> MIRIKDFNHVITGREQPLDINEAIASYITSRYVYFKDARRVAEETWLEAWSLYSGTPEAVDHQRTQTINTVGEVNNDWRHRLNTGKAYECIETVHGYLMGALFPNREWFDLTPNNPGYANEARIIRKYLTKKFNEGKFRVSFEKYLRQLLVCGYSVMALPWRYESRPYKYNVTIKREENEYYDNSTQKANYRTVTENRVTRNAPEFECLDVFDVYLSPTSNDPNESDFIRRIKKTRADIITAIKRGYYTDIDPYDIVNMSAYEVNDRVDKLTSFQGIETNHPYCMDDIIEVVEYWGDLHLDGVSLYDVKATVIGQTLVCCEPNPFWAGKPFVVGSITELPETPYSVGLLQPNMGLLH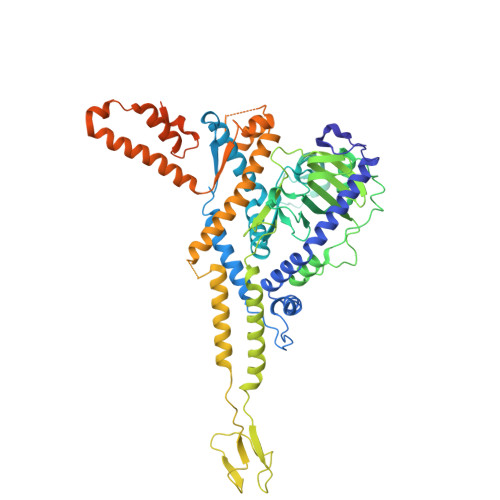QLNIITNQRCDNLELAIDEMWTLVQNSSLNPDEVQVAPGKVFLVDSHDDLRPIQRGGNNFVVSYQEAGLLESTIDRNTGTGNLISANASRSGERVTAAEIQAVRDAGGNRLSNIHRHIEDTSLMEILRRVYRSAQQFVTEPEMIRVSGAKPGEYLFLEVDPESLNKEYSLEPIGADFVTDATKYVRQRMDFIAFASQIPQMAERLNYEALLNDVVNHSGFDDPYSYIVKPQQPAPQPDMGATPEPQTGQAPPDEQTNPFYDIGGVSLQNAIGANIQADGANELINFTTGVNTNADQ>GIE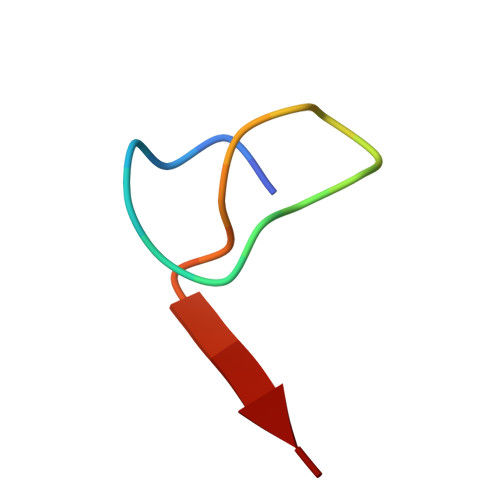PLGPVDEDQGEHYLFAGG[2x]>[2x]MGSSHHHHHHSSGLVPRGSHMASGLYPSYNTSPAAPDSTGMQSTAVQLAGKIRLGWNIGNTMEAIGGETAWGNPMVSNELLKLVKDSGFDAVRIPVAWDQYANQESAEISAAWLNRVKQVVQMAIDNELYVLINIHWDGGWLENNITPAKKDENNAKQKAFWEQIATHLRDFDEHLLFAGTNEPNAENAEQMDVLNSYLQTFVDAVRSTGGKNAYRVLVLQGPVTDIEKTNELWTHMPADTATDRLMAEVHFYTPYNFALMRQDESWGKQFYYWGEGFLSTTDTERNPTWGEEATIDQLFDLMKTKFVDQGIPVVLGEFSAMRRTNLTGDALTLHLAGRAYYHKYVTQQALARGLLPFYWDNGGNDNFSSGIFNRQQNTVFDQQVLDALLEGAGAQ

The highly up-regulated CJA_3010 encodes a signal peptidase II lipoprotein signal peptide (predicted by LipoP 1.0), followed by a serine-rich linker and a GH5_4 catalytic module, and was thus predicted to be anchored extracellularly in the outer membrane by N-terminal cysteine lipidation. Indeed CjGH5D, CjGH5E, and CjGH5F all displayed high specific activity toward XyG. The limit-digest products further revealed that all C. japonicus GH5_4 enzymes specifically catalyze hydrolysis at the anomeric position of the unbranched glucose residues of the (galacto)XyG polysaccharide chain. The overall structure of CjGH5D (residues Gly96 to Gln468) is an (β/α)8 barrel as is typical for GH5 family members.

In contrast, His6-GH5D was produced as a stable, intact, active protein (calculated mass, 44,222.2 Da; observed by ESI–MS, 44,222.6 Da) in excellent yield (150 mg L−1). Despite sequence identities in the 25–40% range, the structure is similar to the catalytic domains of many GH5 enzymes, most of which are annotated as xyloglucanases, glucanases and lichenases, with typical alignment values of approximately 310 residues aligning with an rmsd of 1.3 Å. For example, the structure used for molecular replacement, BoGH5A, overlaps with an r.m.s.d. of 1.1 Å over 332 equivalent Cα atoms with 40% identity. Minor differences are observed between the two structures in loops at the end of core helices.> GSEDFTFDGTKRLSVNYVKGILQPTDTCDIWDKIWNFQAKPDDLLISTYPKAGTTWTQEIVELIQNEGDVEKSKRAPTHQRFPFLEMKIPSLGSGLEQAHAMPSPRILKTHLPFHLLPPSLLEKNCKIIYVARNPKDNMVSYYHFQRMNKALPAPGTWEE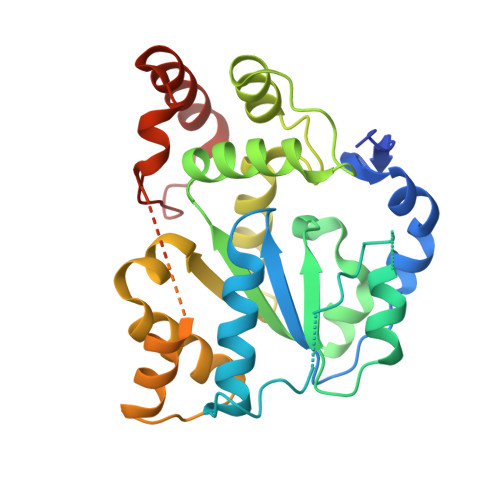YFETFLAGKVCWGSWHEHVKGWWEAKDKHRILYLFYEDMKKNPKHEIQKLAEFIGKKLDDKVLDKIVHYTSFDVMKQNPMANYSSIPAEIMDHSISPFMRKGAVGDWKKHFTVAQNERFDEDYKKKMTDTRLTFHFQF> NKMAMIDLAKLFLASKITAIEFSERICVERRRLYGVKDLSPNILNCGEELFMAAERFEPDADRANYEIDDNGLKVEVRSILEKFKLHHHH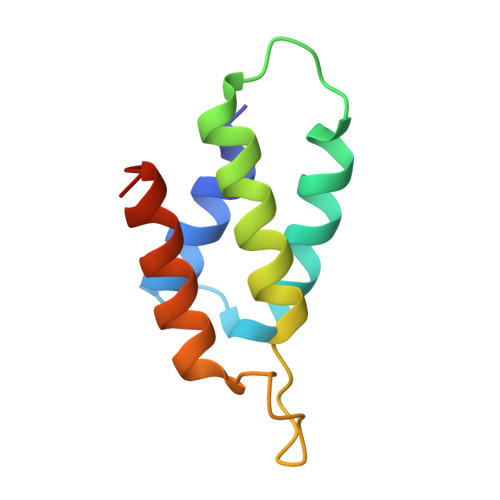H Human dihydroorotate dehydrogenase (hDHODH, EC 1.3.99.11) plays a key role in the de novo pyrimidine biosynthesis. Being located in the inner mitochondrial membrane, it catalyzes the oxidation of dihydroorotate to orotate by involving the cofactor flavin mononucleotide (FMN). This latter is then regenerated by transferring electrons to ubiquinone (coenzyme Q), which is then released in the inner mitochondrial membrane, relating the hDHODH activity to the mitochondrial electron transport chain (ETC). hDHODH inhibitors bind in a tunnel-like pocket, called “lipophilic patch”, which is used by ubiquinone to reach FMN during the enzymatic reaction.

With the aim of experimentally confirming the reliability of the molecular modeling protocol herein applied, as well as the interpretations of the SAR data based on the results of the computational studies, we determined the X-ray structure of hDHODH in complex with compound 4, the most potent derivative of the series. The binding mode observed for compound 4 in its crystallographic complex with the enzyme was perfectly superimposable on that predicted by our computational investigation since all different structural moieties of the inhibitor were found to essentially assume the same position and orientation within the hDHODH binding site in both the model and the X-ray structure. Interestingly, most of the protein residues within the enzyme binding site showed the same orientation in the crystal structure and the model; in fact, all ligand–protein interactions predicted for compound 4 by our modeling studies were experimentally confirmed. Moreover, the ligand forms two different H-bonds with the positively charged guanidine moiety of R136 through both the geminal oxygen and nitrogen of its 2-hydroxypyrazolo[1,5-a]pyridine group that are maintained during almost the whole MD simulation, thus actually establishing a salt bridge interaction with R136. In particular, the 2-hydroxypyrazolo[1,5-a]pyridine moiety, which is negatively charged under physiological conditions, is predicted to present a similar charge density on the oxygen and the geminal nitrogen, thus allowing the ligand to form a charge-assisted H-bond with the side chain of Q47, through its 2-hydroxypyrazolo[1,5-a]pyridine oxygen. Ring A of the ligand is sandwiched between M43 and A59, while its isopropyl substituent is placed in a hydrophobic pocket mainly delimited by M43, L46, L50, A55, and L58, thus forming lipophilic interactions with these residues. Finally, the methyl group connected to ring A makes hydrophobic contacts with F98, L359, and P364, whereas the terminal phenoxyl substituent interacts with Y38 and F62 through aromatic interactions and also makes contact with L68 and P364.

> ATGDERFYAEHLMPTLQGLLDPESAHRLAVRFTSLGLLPRARFQDSDMLEVRVLGHKFRNPVGIAAGFDKHGEAVDGLYKMGFGFVEIGSVTPKPQEGNPRPRVFRLPEDQAVINRYGFNSHGLSVVEHRLRARQQKQAKLTEDGLPLGVNLGKNKTSVDAAEDYAEGVRVLGPLADYLVVNVSSPNTAGLRSLQGKAELRRLLTKVLQERDGLRRVHRPAVLVKIAPDLTSQDKEDIASVVKELGIDGLIVTNTTVSRPAGLQGALRSETGGLSGKPLRDLSTQTIREMYALTQGRVPIIGVGGVSSGQDALEKIRAGASLVQLYTALTFWGPPVVGKVKRELEALLKEQGFGGVTDAIGADHRR> MSVSGVFSKGRGIGHEATTSILRYIPRARVPWQPSRFGRENLTAADMARLWSRGRYRDGPGNYNSGYCTERTHVLEENTVSIIPRRELEKYMPDITIGPKALVTPVSLMNARNGHRVTHDLLHSYDPHIGRLGKPAVVDHDNITVEDPNRVGLNAATLDCRGRIYRWLRRGPFFQVDNYFRRSVKLNRDGTLPTDFVHEAPLMRKIIRLAHRGHLKAACEEYRRVTTVPPVEVYRALTACCVPGAKLADAVSIFEDGDSKLFYVSRDGEVLHNLMRCAIAARHRARIMWVYNVMRGRFYENVVVRAE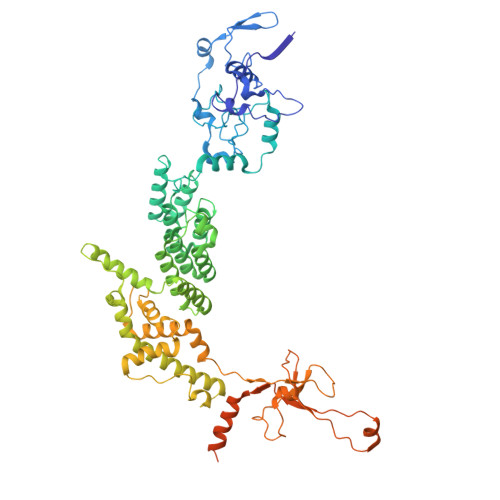VDLIWRYRIAMIALEYLLDHECAEEAAAIYSYLVEEELLRCDVHVRVGLHMREAIAAGKPITLNNDVMNATSLVRDATAVAPEVARELQRRHAQTLQNNAVEAVGAENVREGSAPWSILGPLTAIGPTAEDTMVWLQQHYGDVDVMSIMRWARFRKGKDLMAKDRPQYLARAAAWIELLSKRNREMEEVPLTYMRKSKPLVLDTNSNVRVAWQTPLMRSGGPPRLLAREEGYVFHHSNSSRFVEETYRHPGESLQSRYLALQPLHTEVSAKEDFQRLYYQAQKHHKQQERLLPVSTAAIPSRIVHHSVMSALHGVSGKGEPANRSLFTXNKSNDSHSNTGVASGTSACTDGAGSATPEF>[7x]MSIHFDFKNKQGKELLALNRQWNELSGYRAHAFNESVNMLNNVGETFGVNGANAMQTNMQRVDEMYRLVDSTGTGEDRDWGNQTLLGRLLSQAQTVSIG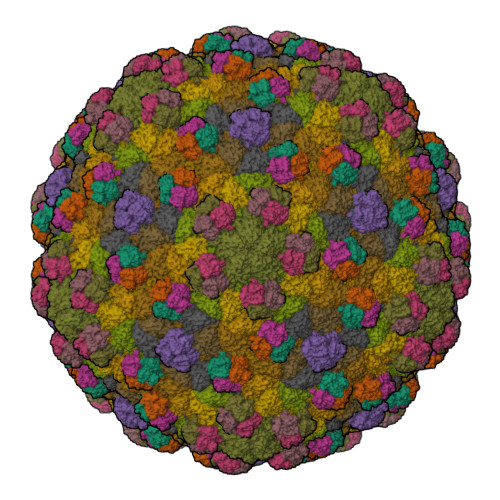KKVIESRRYSEAGRINRSMSGQTDIDMDKTKSSYQKMVIPVFDGAYGRDFRDYEAMRSEMLPALAEDSEEIEFTLLDDVNDYLWNGDAKLKVDTAVWGGLKADASVAAYSLGADLTTATEAQVVAELLALLDVLRITNKKSGPFELYISPQIMSNWQKLAGANTNGFMNIMAAVRALIPEFSVVEADSALQGNQVLCSVVGTRGLHAKIGMMMSSYQVPRVMHNDPYQFVKWFAAGFQSNNSFSGLKSTVYGS;>MANSKNSIFVGGAGRVKQTIEGLAQSAFKPGQLLARAAGDAIDVTAKASTTYGNEFLICDDQPQTLGGGTDVAVTAGDTVQAISVLPGQYVLLSFAATQNVTTKGAAVASNGDGNFKLGNPATEQTFAVTEEIINVTTAGTLVLCRAI[7x]>MKHTVEVMIPEAEIKARIAELGRQITERYKDSGSEMVLVGLLRGSFMFMADLCREVQVPHEVDFMTASSYGSGMSTTRDVKILKDLDEDIRGKDVLIVEDIIDSGNTLSKVREILGLREPKSLAICTLLDKPSRRE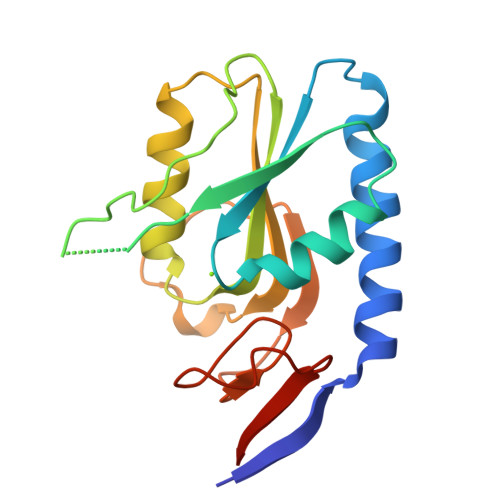VDVPVEFVGFSIPDEFVVGYGIDYAQRYRHLPYVGKVVLLDE[2x]> GSLQLWQFLVTLLDDPANAHFIAWTGRGMEFKLIEPEEVARRWGIQKNRPAMNYDKLSRSLRYY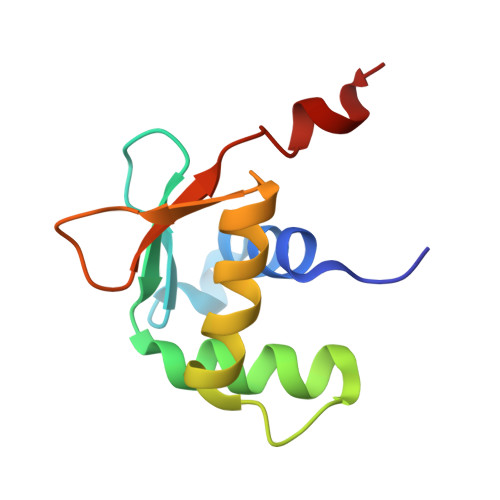YEKGIMQKVAGERYVYKFVCDPDALFSM Here, we report the structural and biochemical studies of the highly conserved C962R protein of ASFV, showing that C962R is a multidomain protein. The N-terminal AEP domain is responsible for the DNA polymerization activity, whereas the DNA unwinding activity is catalyzed by the central SF3 helicase domain. The middle PriCT2 and D5_N domains and the C-terminal Tail domain all contribute to the DNA unwinding activity of C962R. C962R preferentially works on forked DNA, and likely functions in Base-excision repair (BER) or other repair pathway in ASFV.

Using the new variant sample, we also solved one AEP-dCTP-Mn2+ ternary complex structure. The dCTP was captured at the active site of the protein, coordinating tightly with the Mn2+ ions. The A-site Mn2+ coordinates with the non-bridging oxygen atoms from all three phosphate groups, whereas the B-site Mn2+ only coordinates with the α-phosphate group of dCTP. Besides Mn2+ ions, the phosphate groups of dCTP also form H-bond interactions with the side chains of His157 and Tyr221. Binding of dCTP has no obvious impacts on Asp97, Asp99, His157, Asp200 and Tyr221, but it leads to an approximately 100° rotation of the side chain of Tyr83. The Leu21-Val37 region folds into one helix (α2) in the apo-form AEP structure, but it is disordered in the binary and ternary structures of the AEP domain. Superposition shows that the overall folding of the AEP domains is similar in our AEP-dNTP-Mn2+ structure and the HsPrimPol-DNA-dATP complex. Likely, due to the lack of pairing with the template nucleotide, the nucleobase of dCTP in our structure is different from dATP in the HsPrimPol complex; however, the triphosphate groups adopt similar conformations in the two structures. Conservation in catalytic residues, cation-coordination and dNTP binding suggests that C962R may follow a conserved two-cation-assisted mechanism in dNTP incorporation as other primase family proteins.

>[4x]GSLAEVQALETLLARELSVFLTEPGSKKTNIINRITGKTYALPSTELLRFYEHLEQCRKQGALMYFLERQGTYSGLMLDYDLKLNTNAAPSLESSVLSRLCHRIFVHIKNSSVLPEGSHKIHFFFTLKPEAVQGKYGFHVLIPGLKMAASTKKSIIASLQHDATVQKILHEQGVANPESCLDPHSASVPSLLYGSSKLNHRPYQLKTGFELVFDSSDPDYIPIHQIKNIESYNLVSELSLTNEQGSLVRPVYCA> GSHMSEELPQIEIVQEGDNTTFAKPGDTVTIHYDGKLTNGKEFD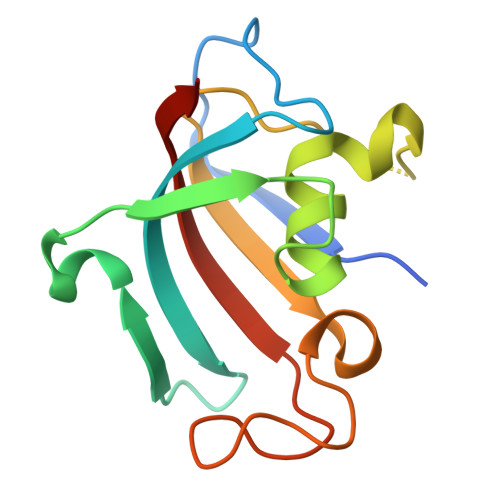SSRKRGKPFTCTVGVGQVIKGWDISLTNNYGKGGANLPKISKGTKAILTIPPNLAYGPRGIPPIIGPNETLVFEVELLGVNGQ> KKAVINGEQIRSISDLHQTLKKELALPEYYGENLDALWDCLTGWVEYPLVLEWRQFEQSKQLTENGAESVLQVFRE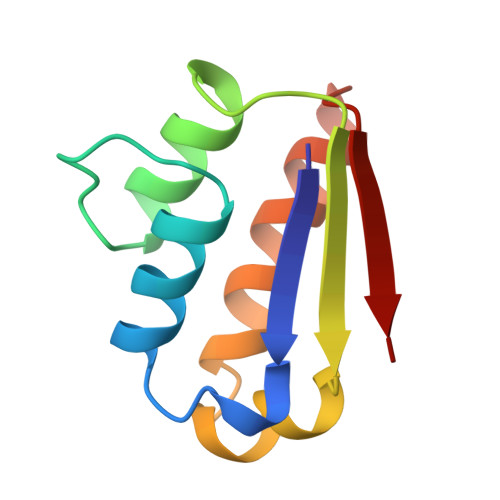AKAEGCDITIILS> MEFTYSYLFRMISHEMKQKADQKLEQLDITNEQGHTLGYLYAHQQDGLTQNDIAKALQRTGPTVSNLLRNLERKKLIYRYVDAQDTRRKNIGLTTSGIKLVE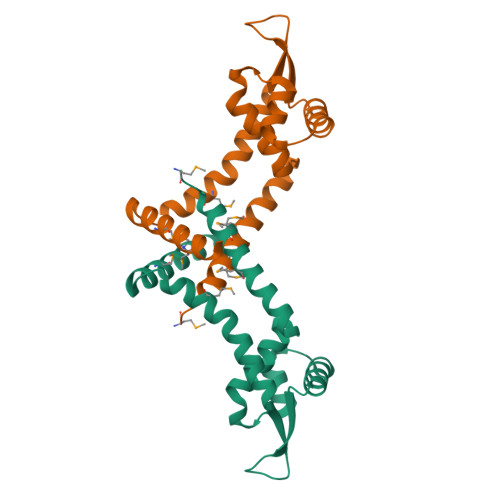AFTSIFDEMEQTLVSQLSEEENEQMKANLTKMLSSLQHHHHHH>[3x]GSHMSLIDPRAIIDPSARLAADVQVGPWSIVGAEVEIGEGTVIGPHVVLKGPTKIGKHNRIYQFSSVGEDTPDLKYKGEPTRLVIGDHNVIREGVTIHRGTVQDRAETTIGDHNLIMAYAHIGHDSVIGNHCILVNNTALA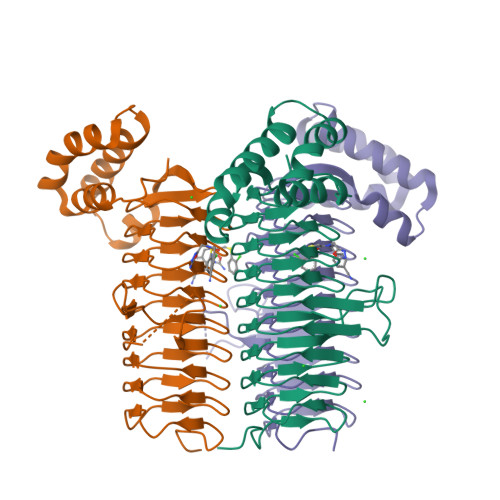GHVHVDDWAILSGYTLVHQYCRIGAHSFSGMGSAIGKDVPAYVTVFGNPAEARSMNFEGMRRRGFSSEAIHALRRAYKVVYRQGHTVEEALAELAESAAQFPEVAVFRDSIQSATRGITR> MDETGKE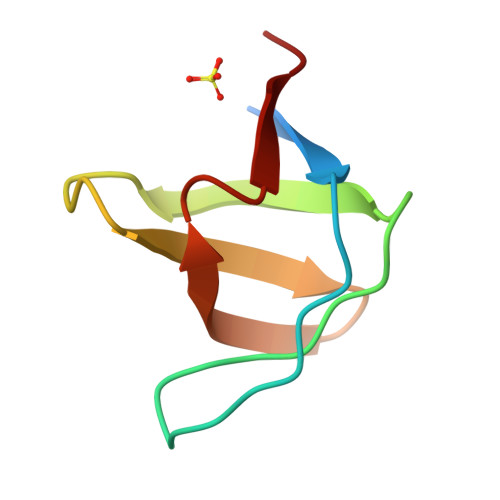LVLALYDYQEKSPAEVTMKKGDILTLLNSTNKDWWKVEVNDRQGFVPAAYVKKLD> MGSSHHHHHHSTGSTEHSCSSQKQISIQHRQTQSDLTIEKISALENSKNSDLEKKEGRIDDLLRANCDLRRQIDEQQKMLEKYKERLNRCVTMSKKLLIEKSKQEKMACRDKSMQDRLRLGHFTTVRHGASFTEQWTDGYAFQNLIKQQERINSQREEIERQRKMLAKRKPPAMGQAPPATNEQKQRKSKTNGAENETPSSGNT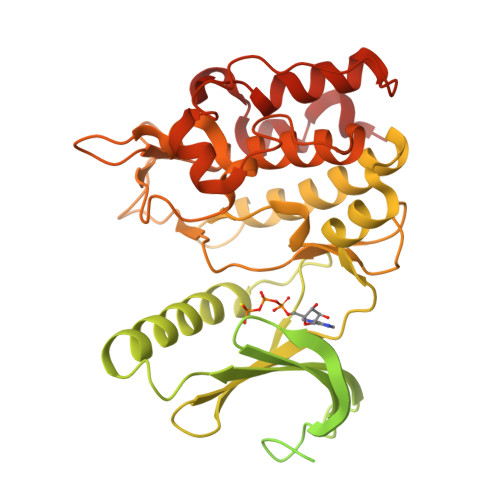ELKDTAPALGAHSLLRLTLAEYHEQEEIFKLRLGHLKKEEAEIQAELERLERVRNLHIRELKRIHNEDNSQFKDHPTLNDRYLLLHLLGRGGFSEVYKAFDLTEQRYVAVKIHQLNKNWRDEKKENYHKHACREYRIHKELDHPRIVKLYDYFSLDTDSFCTVLEYCEGNDLDFYLKQHKLMSEKEARSIIMQIVNALKYLNEIKPPIIHYDLKPGNILLVNGTACGEIKITDFGLSKIMDDDSYNSVDGMELTSQGAGTYWYLPPECFVVGKEPPKISNKVDVWSVGVIFYQCLYGRKPFGHNQSQQDILQENTILKATEVQFPPKPVVTPEAKAFIRRCLAYRKEDRIDVQQLACDPYLLPHIRKSVSTSSPA> GPLGSMSMELFHGSYEEISEIRDSGVFGGLFGAHEKETALSHGETLHRIISPLPLTDYALNYEIESA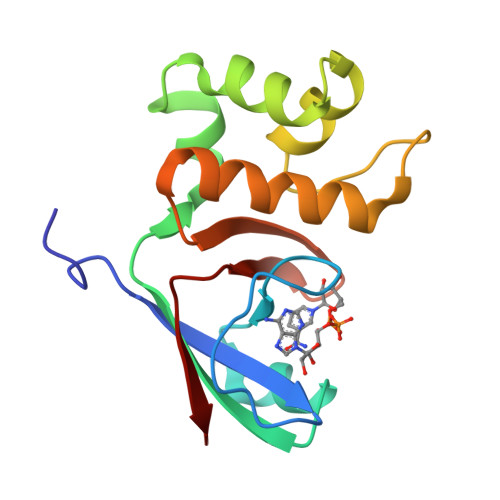WEVALDVAGGDENVAEAIMAKACESDSNDGWELQRLRGVLAVRLGYTSVEMEDEHGTTWLCLPGCTVEKI>[2x]MAKKTSSGSETPDLTVATRTGSKDLPIRNIPGNYGLPIVGPIKDRWDYFYDQGAEEFFKSRIR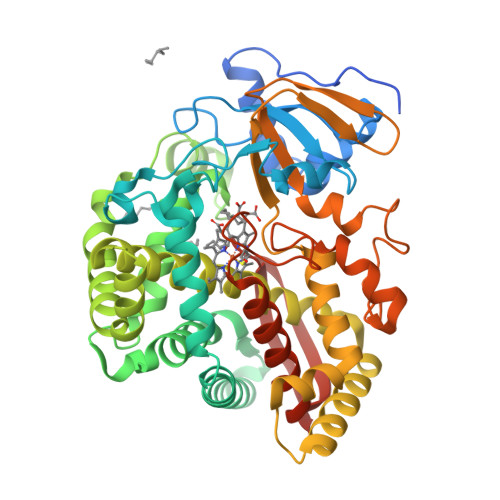KYNSTVYRVNMPPGAFIAENPQVVALLDGKSFPVLFDVDKVEKKDLLTGTYMPSTELTGGYRILSYLDPSEPKHEKLKNLLFFLLKSSRNRIFPEFQATYSELFDSLEKELSLKGKADFGGSSDGTAFNFLARAFYGTNPADTKLKADAPGLITKWVLFNLHPLLSIGLPRVIEEPLIHTFSLPPALVKSDYQRLYEFFLESAGEILVEADKLGISREEATHNLLFATCFNTWGGMKILFPNMVKRIGRAGHQVHNRLAEEIRSVIKSNGGELTMGAIEKMELTKSVVYECLRFEPPVTAQYGRAKKDLVIESHDAAFKVKAGEMLYGYQPLATRDPKIFDRADEFVPERFVGEEGEKLLRHVLWSNGPETETPTVGNKQCAGKDFVVLVARLFVIEIFRRYDSFDIEVGTSPLGSSVNFSSLRKASFHHHH> DPISNAIENAVSTLADTTISRVTAANTAASSHSLGTGRVPALQAAETGASSNASDENLIETRCVMNRNGVNEASVEHFYSRAGLVGVVEVKDSGTSQDGYTVWPIDVMGFVQQRRKLELSTYMRFDAEFTFVSNLNDSTTPGMLLQYMYVPPGAPKPDGRKSYQWQTATNPSIFAKLSDPPPQVSVPFMSPASAYQWFYDGYPTFGEHKQATNLQYGQCPNNMMGHFAIRTVSESTTGKNVHVRVYMRIKHVRAWVPR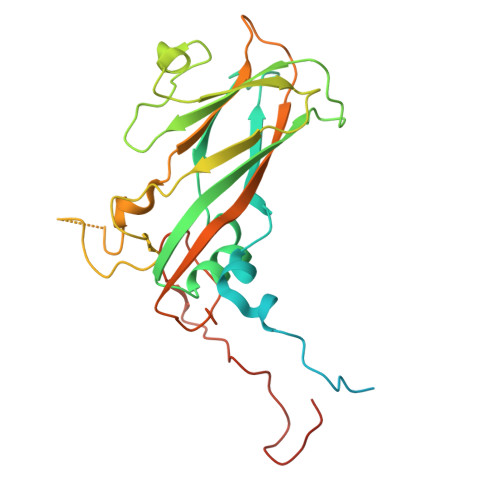PFRSQAYMVKNYPTYSQTISNTAADRASITTTDYEGGVPANPQRTF>[12x]MTVDEQVSNYYDMLLKRNAGEPEFHQAVAEVLESLKIVLEKDPHYADYGLIQRLCEPERQLIFRVPWVDDQGQVHVNRGFRVQFNSALGPYKGGLRFHPSVNLGIVKFLGFEQIFKNSLTGLPIGGGKGGSDFDPKGKSDLEIMRFCQSFMTELHRHIGEYRDVPAGDIGVGGREIGYLFGHYRRMANQHESGVLTGKGLTWGGSLVRTEATGYGCVYFVSEMIKAKGESISGQKIIVSGS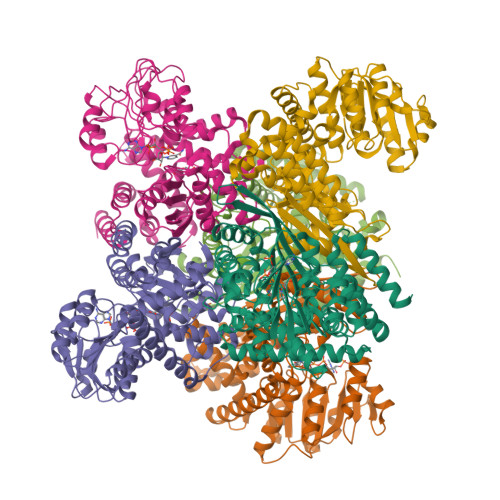GNVATYAIEKAQELGATVIGFSDSSGWVHTPNGVDVAKLREIKEVRRARVSVYADEVEGATYHTDGSIWDLKCDIALPCATQNELNGENAKTLADNGCRFVAEGANMPSTPEAVEVFRERDIRFGPGKAANAGGVATSALEMQQNASRDSWSFEYTDERLQVIMKNIFKTCAETAAEYGHENDYVVGANIAGFKKVADAMLAQGVI>MLNTTFANAKFANPFMNASGVHCMTIEDLEELKASQAGAYITKSSTLEKREGNPLARYVDLELGSINSMGLPNLGFDYYLDYVLKNQKENAQEGPIFFSIAGMSAAENIAMLKKIQESDFSGITELNLSCPNVPGKPQLAYDFEATEKLLKEVFTFFTKPLGVKLPPYFDLVHFDIMAEILNQFPLTYVNSVNSIGNGLFIDPEAESVVIKPKDGFGGIGGAYIKPTALANVRAFYTRLKPEIQIIGTGGIETGQDAFEHLLCGATMLQIGTALHKEGPAIFDRIIKELEEIMNQK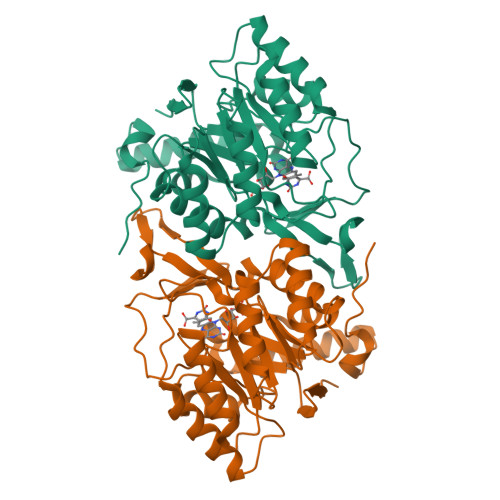GYQSIADFHGKLKSL[2x]> GAMGSVNIPRKEKDFQGMLEYKKEDEQKLVKNLILELKPRGVAVNLIPGLPAYILFMCVRHADYLNDDQKVRSLLTSTINSIKKVLKKRGDDFETVSFWLSNTCRFLHC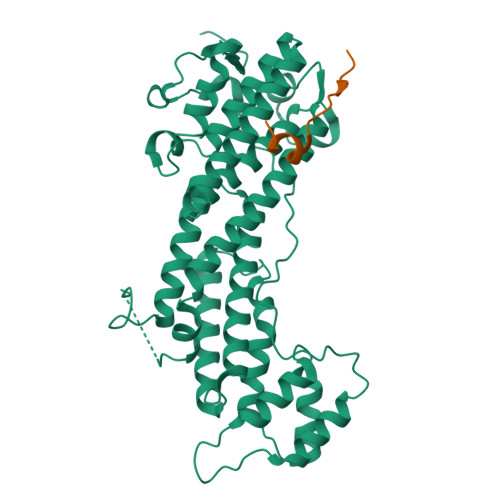LKQYSGEEGFMKHNTSRQNEHCLTNFDLAEYRQVLSDLAIQIYQQLVRVLENILQPMIVSGMLEHETIQGVSGVKPTGLRKRTSSIADEGTYTLDSILRQLNSFHSVMCQHGMDPELIKQVVKQMFYIIGAITLNNLLLRKDMCSWSKGMQIRYNVSQLEEWLRDKNLMNSGAKETLEPLIQAAQLLQVKKKTDDDAEAICSMCNALTTAQIVKVLNLYTPVNEFEERVSVSFIRTIQMRLRDRKDSPQLLMDAKHIFPVTFPFNPSSLALETIQIPASLGLGFISRV;> QRPRPRVLLKAPTLAEMEEMNTSEEEE>MFHSSAMVNSHRKPMFNIHRGFYCLTAILPQICICSQFSVPSSYHFTEDPGAFPVATNGERFPWQELRLPSVVIPLHYDLFVHPNLTSLDFVASEKIEVLVSNATQFIILHSKDLEITNATLQSEEDSRYMKPGKELKVLSYPAHEQIALLVPEKLTPHLKYYVAMDFQAKLGDGFEGFYKSTYRTLGGETRILAVTDFEPTQARMAFPCFDEPLFKANFSIKIRRESRHIALSNMPKVKTIELEGGLLEDHFETTVKMSTYLVAYIVCDFHSLSGFTSSGVKVSIYASPDKRNQTHYALQASLKLLDFYEKYFDIYYPLSKLDLIAIPDFAPGAMENWGLITYRETSLLFDPKTSSASDKLWVTRVIAHELAHQWFGNLVTMEWWNDIWLNEGFAKYMELIAVNATYPELQFDDYFLNVCFEVITKDSLNSSRPISKPAETPTQIQEMFDEVSYNKGACILNMLKDFLGEEKFQKGIIQYLKKFSYRNAKNDDLWSSLSNSCLESDFTSGGVCHSDPKMTSNMLAFLGENAEVKEMMTTWTLQKGIPLLVVKQDGCSLRLQQERFLQGVFQEDPEWRALQERYLWHIPLTYSTSSSNVIHRHILKSKTDTLDLPEKTSWVKFNVDSNGYYIVHYEGHGWDQLITQLNQNHTLLRPKDRVGLIHDVFQLVGAGRLTLDKALDMTYYLQHETSSPALLEGLSYLESFYHMMDRRNISDISENLKRYLLQYFKPVIDRQSWSDKGSVWDRMLRSALLKLACDLNHAPCIQKAAELFSQWMESSGKLNIPTDVLKIVYSVGAQTTAGWNYLLEQYELSMSSAEQNKILYALSTSKHQEKLLKLIEL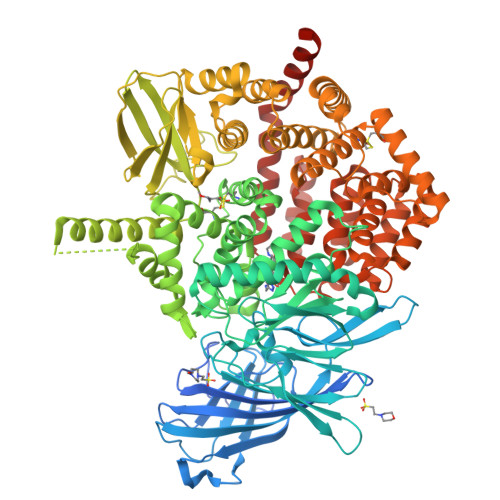GMEGKVIKTQNLAALLHAIARRPKGQQLAWDFVRENWTHLLKKFDLGSYDIRMIISGTTAHFSSKDKLQEVKLFFESLEAQGSHLDIFQTVLETITKNIKWLEKNLPTLRTWLMVNTRHHHHHH[2x]> DNIEDIPLGSSEQDPYDFFTLSDRNVMNSDMKKNIVQWNSRYSYNQLKNKDSLIMFLVEIFRSLFVSNCIDKNIDNVLLSIEEMFIDHYYNPQHSRLKYLIDDVGIFFTKLPITKAFHTYNKKYRITKRLYAPPTFNEVRHILNLAQILSLEEGLDLLTFDADETLYPDGHDFNDEVLASYISCLLKKMNIAIVTAASYNNDAEKYQKRLENLLKYFSKHNIKDGSYKNFYVMGGESNYLFKCNEEATLYSVPENEWRHYKKFVDYDTVQEILNISEKCLEKVIKDFGLCAQIQRKEKSIGLVPNKIPSLNIKNEQKNYMIKYEVLEEAVIRIKKEIIKNKITAPYCAFNGGQDLWVDVGNKAEGLLILQKLLKIQKKKCCHIGDQFLHSGNDFPTRFCSLTLWVSNPQETKACLKSIMHLNIKSFIPEVLYENQ;> KDSLIMFLVEIFRSLFVSNCIDKNIDNVLLSIEEMFIDHYYNPQHSRLKYLIDDVGIFFTKLPITKAFHTYNKKYRITKRLYAPPTFNEVRHILNLAQILSLEEGLDLLTFDADETLYPDGHDFNDEVLASYISCLLKKMNIAIVTAASYNNDAEKYQKRLENLLKYFSKHNIKDGSYKNFYVMGGESNYLFKCNEEATLYSVPENEWRHYKKFVDYDTVQEILNISEKCLEKVIKDFGLC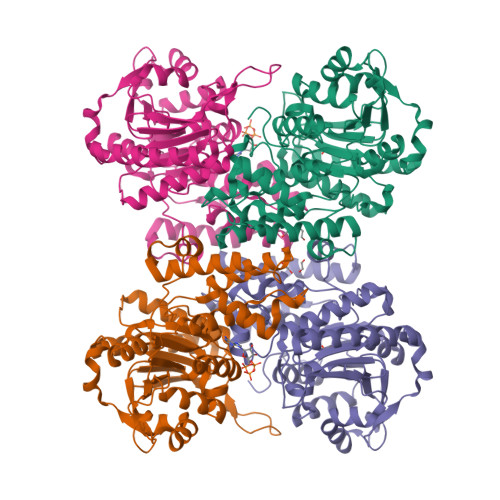AQIQRKEKSIGLVPNKIPSLNIKNEQKNYMIKYEVLEEAVIRIKKEIIKNKITAPYCAFNGGQDLWVDVGNKAEGLLILQKLLKIQKKKCCHIGDQFLHSGNDFPTRFCSLTLWVSNPQETKACLKSIMHL>[2x]MHHHHHHSSGRENLYFQGNTTKHIILVRHGQYERRYKDDENSKRLTKEGCKQADITGKKLKDILNNKKVSVIYHSDMIRAKETANIISKYFPDANLINDPNLN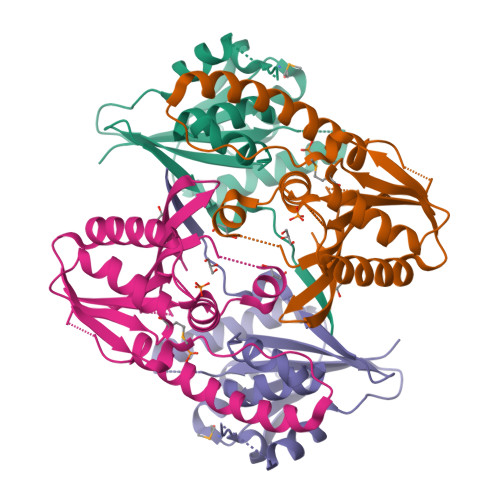EGTPYLPDPLPRHSKFDAQKIKEDNKRINKAYETYFYKPSGDEDEYQLVICHGNVIRYFLCRALQIPLFAWLRFSSYNCGITWLVLDDEGSVVLREFGSVSHLPFESVTYF>[2x]FEFPEELKTKLQEHINYFPKKRQAILLCLHEIQNYYGYIPPESLKPLADMLELPLNHVEGVVAFYDMFDREDKAKYRIRVCVSIVCHLMGTNKLLKALENILGIKPGEVTPDGKFKIVPVQCLGACSEAPVFMVNDDEYKFESEVQLNEILSRYT;>RSYPAIPRIYAETTLNMLLKRAKKPRVHSIDEYLKDGGYQALEKALNMSPEEIIDWVDKSTLRGRGGAGFPTGKKWKFAVQNPGPRYFICNADESEPGTFKDRIIIERDPHLLIEGIIISSYAIGANEAYIYIRGEYPAGYYILRDAIEEAKKKGFLGKNILGSGFDLEIYVARGAGAYICGEETALIESLEGKRGHPRLKPPYPVQKGLWGKPTVVNNVETIANVPFIISMGWEEYRYIGPSDYAGPKLFPVSGKVKKPGVYELPMNTTLREVIFKYAGGTLGNKKVKAVFSGALDCFSSEE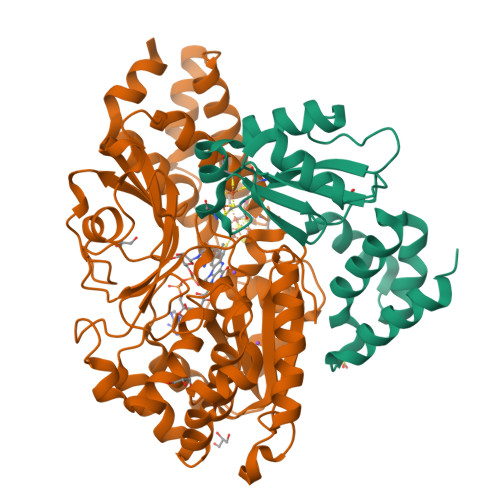LDIPMDYSPLGFGGTGTVIVLTEEDDIVEAALKIAEFYEHETCGQCTPCRVGCYEQANLLEKIYKGEATEQDWEGFDFVNRNIQPTSICGLGAVAGRLIRQTLEKFPEEWEKYRK[2x]> MGAQVSTQKTGAHETGLNASGNSIIHYTNIN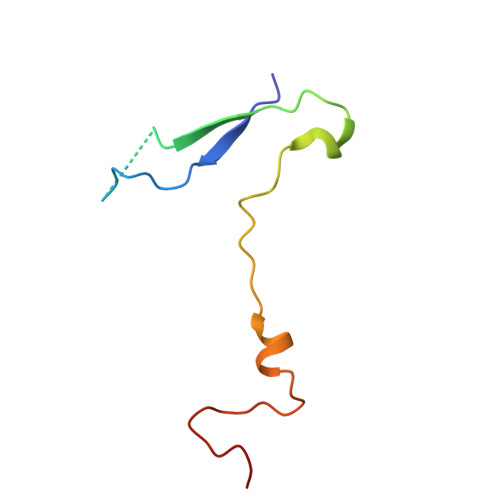YYKDAASNSANRQDFTQDPGKFTEPVKDIMIKTMPALNS> MSKGASAPQQQSAFKQLYTELFNNEGDFSKVSSNLKKPLKCYVKESYPHFLVTDGYFFVAPYFTKEAVNEFHAKFPNVNIVDLTDKVIVINNWSLELRRVN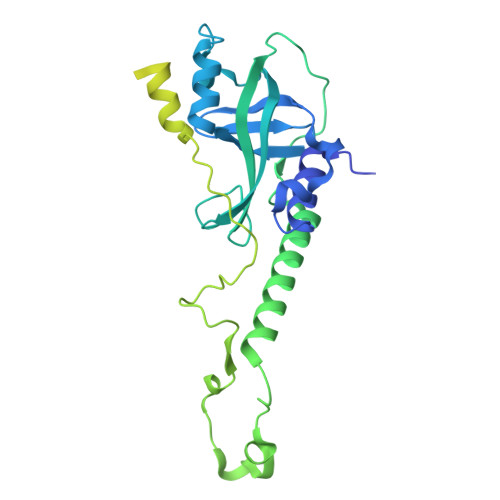SAEVFTSYANLEARLIVHSFKPNLQERLNPTRYPVNLFRDDEFKTTIQHFRHTALQAAINKTVKGDNLVDISKVADAAGKKGKVDAGIVKASASKGDEFSDFSFKEGNTATLKIADIFVQEKGKDALNKAADHTDGAKVKGGAKGKGKAAAKAAKGKKLSAKKGDSSAADVRKSVDKIVKYTPSKGSRKDTPQKSQAPAAGKSSAKKGGKKAVPSAPSPSGKKSALTTDKMTMAQFVKYLDWHEKKKGGKVSSGGKVLGKRSAGKASATSGKASKASKKTAAKK The flavin adenine dinucleotide (FAD)-dependent glucose dehydrogenases (FADGDHs; EC 1.1.5.9) comprise oxidoreductases that catalyze the oxidation of first hydroxyl group of glucose and other sugar molecules, using FAD as the primary electron acceptor (systematic name; D-glucose:acceptor 1-oxidoreductase). Recently, fungus-derived FADGDH has received attention as the enzyme for glucose monitoring, especially self-monitoring of blood glucose (SMBG), exploiting its oxygen insensitivity and narrow substrate specificity, in particular its lack of activity toward maltose. The structure of AfGDH consists of two major domains: an FAD-binding domain and a C-terminal domain. The overall structure was found to be similar to that of the fungal GOxs reported till date.

We obtained the X-ray structures of binary complex of enzyme and reduced FAD at a resolution of 1.78 Å, and the ternary complex with reduced FAD and D-glucono-1,5-lactone (LGC) at a resolution of 1.57 Å. The bound FAD molecule was refined as a reduced FAD cofactor (FADH2), observed not only in AfGDH/LGC but also in AfGDH alone. Both FAD molecules showed clear electron density maps for bending of the isoalloxazine ring of reduced FAD. In the structure of AfGDH alone, we could not identify the bent isoalloxazine ring conformation showing the hydroquinone or semiquinone state, but it clearly shows a bend, as observed in AfGDH/LGC, and was refined as reduced FAD. The subunit structure of AfGDH is similar to that of AnGOx and PaGOx, but the recombinant AfGDH is unlikely to form a dimer conformation, according to PISA39. In fact, size exclusion chromatography analysis of AfGDH revealed that recombinantly prepared nonglycosylated AfGDH eluted at an elution volume corresponding to its monomer, unlike GOx, which is eluted at an elution volume corresponding to its dimer. The β turn between B10 and B11 of AfGDH is directed toward the N-terminal region containing a short α helix of GOxs and is located between the N-terminal region and the corresponding β turn of GOxs. The observed position of the β turn in recombinant AfGDH is expected to prevent dimer formation due to the steric hindrance at the most plausible dimer interface (Supplementary Figure S5 (b)). Unlike in GOxs, no residues from AfGDH belonging to the loop between B4 and H7 lie near the active site, and a cavity is present in the vicinity of the substrate-binding site.

> MNTTTYDYIVVGGGTSGLVVANRLSENPDVSVLLLEAGASVFNNPDVTNANGYGLAFGSAIDWQYQSINQSYAGGKQQVLRAGKALGGTSTINGMAYTRAEDVQIDVWQKLGNEGWTWKDLLPYYLKSENLTAPTSSQVAAGAAYNPAVNGKEGPLKVGWSGSLASGNLSVALNRTFQAAGVPWVEDVNGGKMRGFNIYPSTLDVDLNVREDAARAYYFPYDDRKNLHLLENTTANRLFWKNGSAEEAIADGVEITSADGKVTRVHAKKEVIISAGALRSPLILELSGVGNPTILKKNNITPRVDLPTVGENLQDQFNNGMAGEGYGVLAGASTVTYPSISDVFGNETDSIVASLRSQLSDYAAATVKVSNGHMKQEDLERLYQLQFDLIVKDKVPIAEILFHPGGGNAVSSEFWGLLPFARGNIHISSNDPTAPAAINPNYFMFEWDGKSQAGIAKYIRKILRSAPLNKLIAKETKPGLSEIPATAADEKWVEWLKANYRSNFHPVGTAAMMPRSIGGVVDNRLRVYGTSNVRVVDASVLPFQVCGHLVSTLYAVAERASDLIKEDAKSA>GAMDGIYSASGIDVMGILLRIASRPNPTIDLGPLDCSVSLTLCDISLPDAPIVYASPGFYQLTGYSAPEIMGRNCRFLQNSPHMPPPGRVSDAVQEMRRAIRAHQ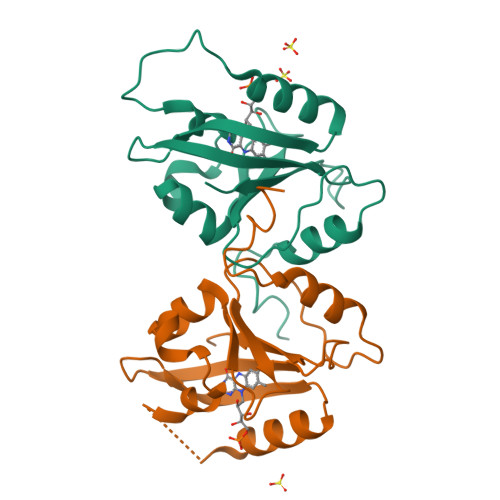EVQVRIVNYKKNGTPFTNVVTILPLWADPSGHHFAVGLQAEL[4x]>[3x]MANVDEAILKRVKGWAPYVDAKLGFRNHWYPVMFSKEINEGEPKTLKLLGENLLVNRIDGKLYCLKDRCLHRGVQLSVKVECKTKSTITCWYHAWTYRWEDGVLCDILTNPTSAQIGRQKLKTYPVQEAKGCVFIYLGDGDPPPLARDTPPNFLDDDMEILGKNQIIKSNWRLAVENGFDPSHIYIHKDSILVKDNDLALPLGFAPGGDRKQQTRVVDDDVVGRKGVYDLIGEHGVPVFEGTIGGEVVREGAYGEKIVANDISIWLPGVLKVNPFPNPDMMQFEWYVPIDENTHYYFQTLGKPCANDEERKKYEQEFESKWKP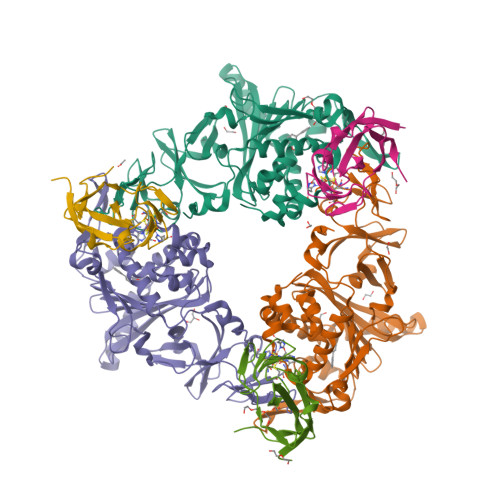MALEGFNNDDIWAREAMVDFYADDKGWVNEILFESDEAIVAWRKLASEHNQGIQTQAHVSGLEHHHHHH;>[3x]MNQIWLKVCAASDMQPGTIRRVNRVGAAPLAVYRVGDQFYATEDTCTHGIASLSEGTLDGDVIECPFHGGAFNVCTGMPASSPCTVPLGVFEVEVKEGEVYVAGEKKLEHHHHHH>[2x]ERGVCACPRIYMPVCGSNLKTYNNDCLLRCEINSDLGRANNLRKIA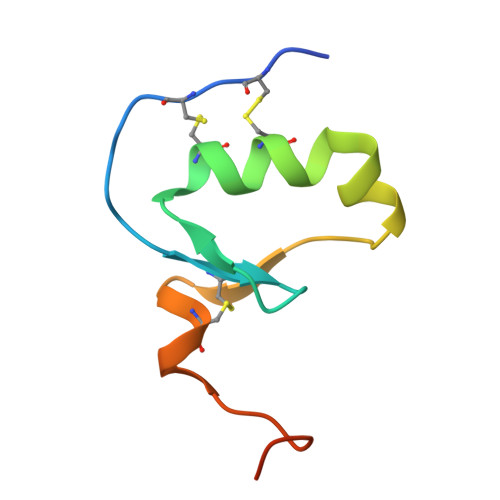DQACDNLTDNVNDFIPQEY1-alpha-hydroxy-vitamin 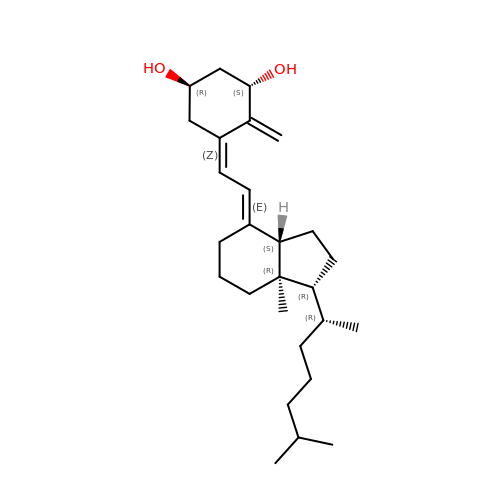D3 | C27 H44 O2 | OFHCOWSQAMBJIW-AVJTYSNKSA-N>[2x]AIGPVTDLTISNADVTPDGFTRAAVVANGVFPGPLITGNKGDNFQINVIDNLTNATMLKTTTIHWHGLFQHGTNWADGPAFVNQCPIASGNSFLYDFTVPDQAGTFWYHSHLSTQYCDGLRGPLVVYDPSDPYASMYDVDDDTTVITLSDWYHTAAKLGPAFPP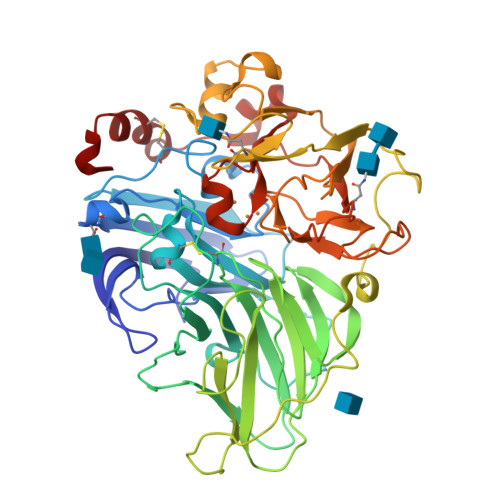NADSVLINGLGRFAGGNASDLAVITVEQNKRYRFRLVSLSCDPNFTFSIDGHNMTIIEVDGVNHEPLEVDSIQIFASQRYSFVLNATQSVDNYWIRAIPNTGTIDTTGGLNSAILRYSGADIVDPTANATTSVIPLVETDLVPLDSPAAPGDPVVGGVDLAMNLDFSFNGTNFFINNETLIPPTVPVLLQILSGAQSASDLLPTGSVYTLPLNSTIELSFPITTVNGVTNAPGAPHPFHLHGHAFSVVRSAGSSDYNYVNPVRRDTVSTGNPGDNVTIRFTTDNAGPWFLHCHIDFHLEAGFAIVFAEDTPDTASVNPVPTAWSDLCPTYDALDPSDH> MHHHHHHARATGKTFRSGNSEAVRLPRDLAFGADVELTLIRSGDV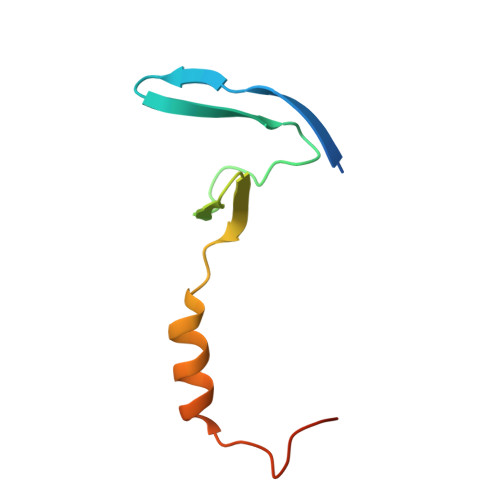LTIYPSKGSIADLVATLNQMPRPDSVEIRDEDL>[4x]MAKKTSSKGKLPPGPLPLPGLGNLLHVDFQNTPYCFDQLRRRFGDVFSLQLAWTPVVVLNGLAAVREALVTHGEDTADRPPVPITQILGFGPRSQGVFLARYGPAWREQRRFSVSTLRNLGLGKKSLEQWVTEEAACLCAAFANHSGRPFRPNGLLDKAVSNVIASLTCGRRFEYDDPRFLRLLDLAQEGLKEESGFLREVLNAVPVLLHIPALAGKVLRFQKAFLTQLDE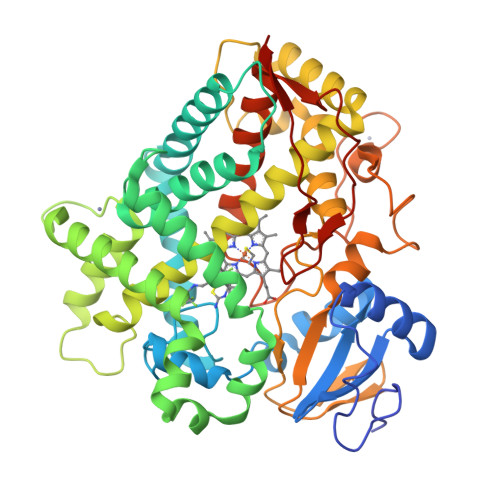LLTEHRMTWDPAQPPRDLTEAFLAEMEKAKGNPESSFNDENLRIVVADLFSAGMVTTSTTLAWGLLLMILHPDVQRRVQQEIDDVIGQVRRPEMGDQAHMPYTTAVIHEVQRFGDIVPLGVTHMTSRDIEVQGFRIPKGTTLITNLSSVLKDEAVWEKPFRFHPEHFLDAQGHFVKPEAFLPFSAGRRACLGEPLARMELFLFFTSLLQHFSFSVPTGQPRPSHHGVFAFLVSPSPYELCAVPRHHHH>[8x]MGREEPLNHVEAERQRREKLNQRFYALRAVVPNVSKMDKASLLGDAIAYINELKS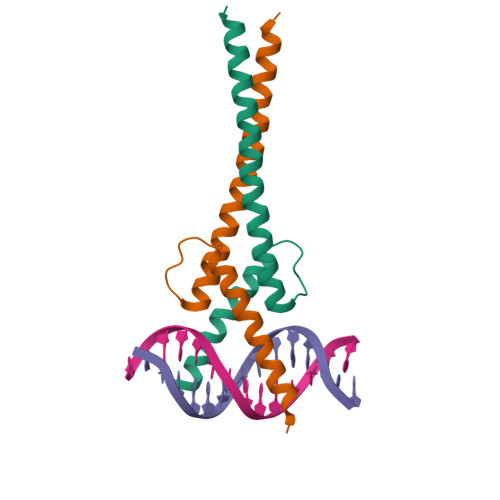KVVKTESEKLQIKNQLEEVKLELAGRLEHHHHHH>MNRVTNLLAWAGAIGLAQATCPFADPAALYSRQDTTSGQSPLAAYEVDDSTGYLTSDVGGPIQDQTSLKAGIRGPTLLEDFMFRQKIQHFDHERVPERAVHARGAGAHGTFTSYADWSNITAASFLNATGKQTPVFVRFSTVAGSRGSADTARDVHGFATRFYTDEGNFDIVGNNIPVFFIQDAIQFPDLIHSVKPRPDNEIPQAATAHDSAWDFFSQQPSTMHTLFWAMSGHGIPRSYRHMDGFGVHTFRFVKDDGSSKLIKWHFKSRQGKASLVWEEAQVLSGKNADFHRQDLWDAIESGNGPEWDVCVQIVDESQAQAFGFDLLDPTKIIPEEYAPLTKLGLLKLDRNPTNYFAETEQVMFQPGHIVRGIDFTEDPLLQGRLFSYLDTQLNRNGGPNFEQLPINMPRVPIHNNNRDGAGQMFIHRNKYPYTPNTLNSGYPRQANQNAGRGFFTAPGRTASGALVREVSPTFNDHWSQPRLFFNSLTPVEQQFLVNAMRFEISLVKSEEVKKNVLTQLNRVSHDVAVRVAAAIGLGA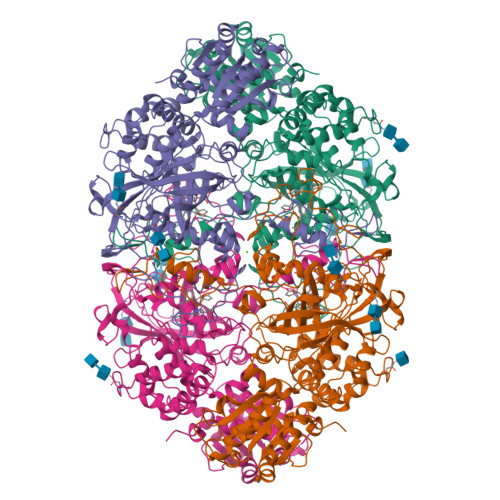PDADDTYYHNNKTAGVSIVGSGPLPTIKTLRVGILATTSESSALDQAAQLRTRLEKDGLVVTVVAETLREGVDQTYSTADATGFDGVVVVDGAAALFASTASSPLFPTGRPLQIFVDAYRWGKPVGVCGGKSSEVLDAADVPEDGDGVYSEESVDMFVEEFEKGLATFRFTDRFALDS[4x]(2R)-N-hydroxy-2-methyl-2-(methylsulfonyl)-4-(2-oxo-4-phenylpyridin-1(2H)-yl)butanamide | 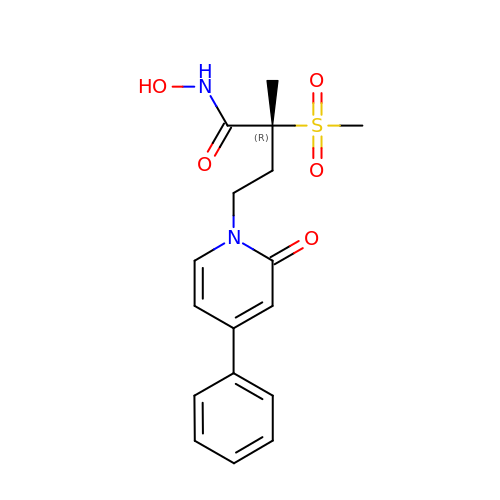C17 H20 N2 O5 S | NFQOWMXNJNMRTA-QGZVFWFLSA-N>[2x]HHHHHHS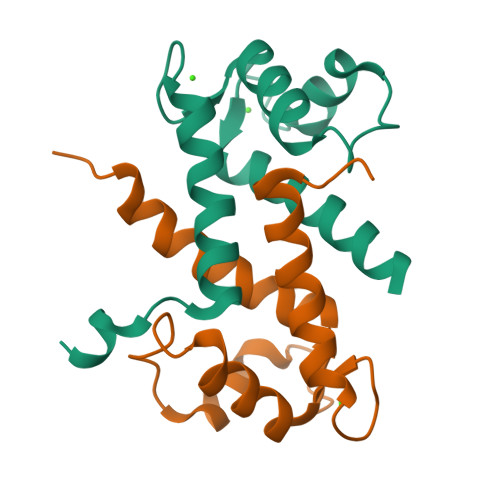LMAAEPLTELEESIETVVTTFFTFARQEGRKDSLSVNEFKELVTQQLPHLLKDVGSLDEKMKSLDVNQDSELKFNEYWRLIGELAKEIRKKKDLKIRKK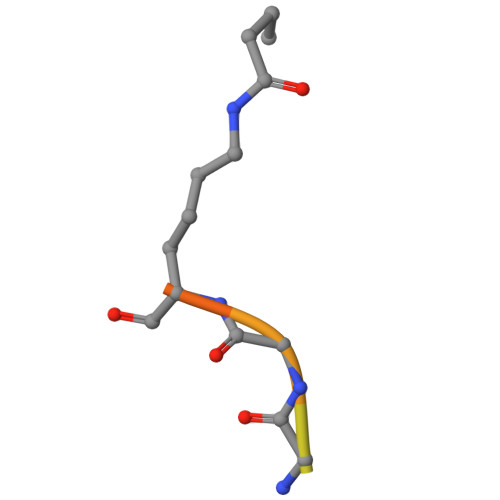> SGRGXGGXGLG> TPRIVIIGAGIVGTNLADELVTRGWNNITVLDQGPLNMPGGSTSHAPGLVFQTNPSKTMASFAKYTVEKLLSLTEDGVSCFNQVGGLEVATTETRLADLKRKLGYAAAWGIEGRLLSPAECQELYPLLDGENILGGLHVPSDGLASAARAVQLLIKRTESAGVTYRGSTTVTGIEQSGGRVTGVQTADGVIPADIVVSCAGFWGAKIGAMIGMAVPLLPLAHQYVKTTPVPAQQGRNDQPNGARLPILRHQDQDLYYREHGDRYGIGSYAHRPMPVDVDTLGAYAPETVSEHHMPSRLDFTLEDFLPAWEATKQLLPALADSEIEDGFNGIFSFTPDGGPLLGESKELDGFYVAEAVWVTHSAGVAKAMAELLTTGRSETDLGECDITRFEDVQLTPEYVSETSQQNFVEIYDVLHPLQPRLSPRNLRVSPFHARHKELGAFFLEAGGWERPYWFEANAALLKEMPAEWLPPARDAWSGMFSSPIAAAEAWKTRTAVAMYDMTPLKRLEVSGPGALKLLQELTTADLAKKPGAVTYTLLLDHAGGVRSAITVARLSEDTFQLGANGNIDTAYFERAARHQTQSGSATDWVQVRDTTGGTCCIGLWGPLARDLVSKVSDDDFTNDGLKYFRAKNVVIGGIPVTAMRLSYVGELGWELYTSADNGQRLWDALWQAGQPFGVIAAGRAAFSSLRLEKGYRSWGTDMTTEHDPFEAGLGFAVKMAKESFIGKGALEGRTEEASARRLRCLTIDDGRSIV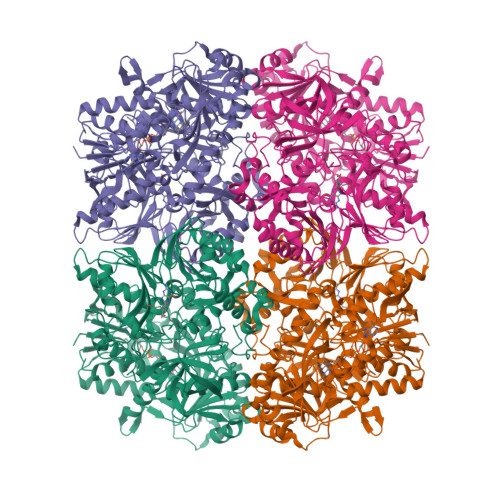LGKEPVFYKEQAVGYVTSAAYGYTVAKPIAYSYLPGTVSVGDSVDIEYFGRRITATVTEDPLYDPKMTRLRG> MDAHAINERYVGPRCHRLAHVVLPRTFLLHHAIPLEPEIIFSTYTRFSRSPGSSRRLVVCGKRVLPGEENQLASSPSGLALSLPLFSHDGNFHPFDISVLRISCPGSNLSLTVRFLYLSLVVAMGAGRNNARSPTVDGVSPPEGAVAHPLEELQRLARATPDPAPTRGPLQVLTGLLRAGSDGDRATHHMALEAPGTVRGESLDPPVSQKGPARTRHRPPPVRLSFNPVNADVPATWRDATNVYSGAPYYVCVYERGGRQEDDWLPIPLSFPEEPVPPPPSLVFMDDLFINTKQCDFVDTLEAACRTQGYTLRQRVPVAIPRDAEIADAVKSHFLEACLVLRGLASEA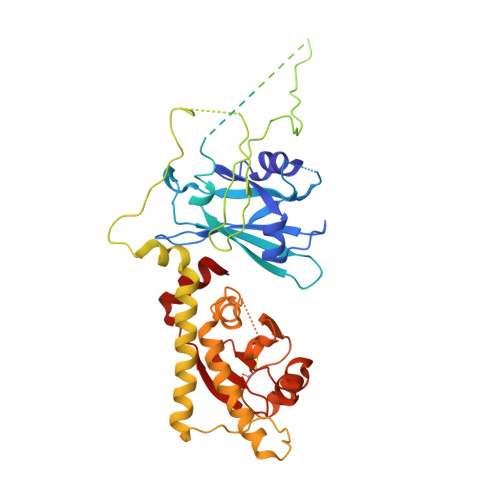SAWIRAATSPPLGRHACWMDVLGLWESRPHTLGLELRGVNCGGTDGDWLEILKQPDVQKTVSGSLVACVIVTPALEAWLVLPGGFAIKGRYRASKEDLVFIRGRYG>DRHHHHHHKLSVPSEDQPGDSYSHGQSCLGCVVLVSVIEQLAEVHNSSVQVAMERLCSYLPEKLFLKTACYFLVQTFGSDIIKLLDEAMKADVVCYALEFCKRGAVQPQCHLYPLPQEAWESALEKARQVLRRSSTMKYRRSGRNICSLPFLTKICQKIELSIKKAVPFKDVDSDKHSVFPTLRGYHWRGRDCNDSDKTVYPGRRPDNWDIHQDSNCNGIWGIDPKDGIPYEKKFCEGSQPRGIILLGDAAGAHFHIPPEWLTASQMSVNSFLNLPSALTDELNWPQLSGVTGFLDSTSGIEEKSIYHRLRKRNHCNHRDYQSISKNGASSRNLKNFIESLSRNQASDHPAIVLYAMIGNDVCNSKADTVPEMTTPEQMYANVMQTLTHLNSHLPNGSHVILYGLPDGTFLWDSLHNRYHPLGQLNKDVTYAQFFSFLRCLQLNPCNGWMSSNKTLRTLTSERAEQLSNTLKKIATTETFANFDLFYVDFAFHEIIEDWQKRGGQPWQLIEPVDGFHPNEVASLLQANRVWEKIQL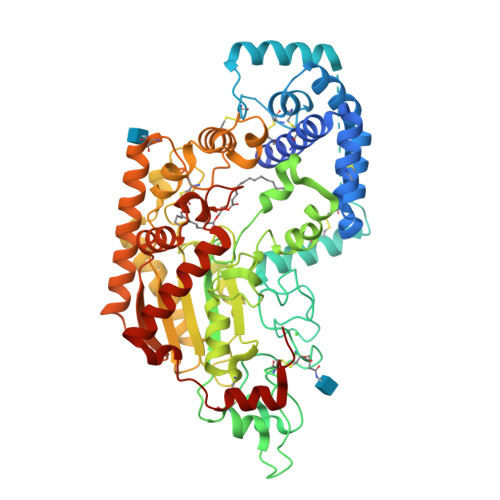QWPHVLGKENPFNSQIEEVFGDQGGH[2x]>MDKAKRNIKPFDGEKYAIWKFRIRALLAEQDVLKVVDGLMPNEVDDSWKKAERCAKSTIIEYLSDSFLNFATSDITARQILENLDAVYERKSLASQLALRKRLLSLKLSSEMSLLSHFHIFDELISELLAAGAKIEEMDKISHLLITLPSCYDGIITAIETLSEENLTLAFVKNRLLDQEIKIKNDHNDTSKKVMNAIVHNNNNTYKNNLFKNRVTKPKKIFKGNSKYKVKCHHCGREGHIKKDCFHYKRILNNKNKENEKQVQTATSHG[9x]

Here, we show that the Ty1 retrotransposon Copia forms virus-like capsids in vivo and transfers between cells. Copia is enriched at the Drosophila neuromuscular junction (NMJ) and transported across synapses, and disrupting its expression promotes both synapse development and structural synaptic plasticity. Because Copia behaves in a viral-like manner, we used cryogenic-electron microscopy (cryo-EM) to determine the high-resolution structure of the Copia capsid and found that it is distinct from the related dArc1 capsid, with a larger internal capacity and the presence of pores similar to those used by retroviruses to carry out their reverse transcriptase activity. The capsid layer is composed of the Copiagag protein’s CA region, which contains 2 alpha-helical domains.

Our purification protocol enriched capsids of sufficient homogeneity such that we could determine their structure using single-particle cryo-EM methods. Our reconstruction of the Copiagag capsid when enforcing T = 9 icosahedral symmetry reached ~4.2-Å overall resolution. There is a layer of featureless density lining the inner surface of the Copia capsid that likely represents the RNA that comigrates with the Copia-gag protein. Because the RNA does not adopt T = 9 symmetry, its density is amorphous in our reconstruction. The NC region is not clearly visualized in the map but is located in the interior of the capsid and is associated with the density attributed to RNA. The Copia capsid is much larger than that of the T = 4 dArc1 capsid (inner radii of ~220 Å and ~170 Å, respectively), resulting in ~2.2× increased internal capacity. We hypothesize that the Copia capsid is larger than dArc1 because it packages larger cargo, such as the longer Copia mRNA (5 kbp versus 2 kbp) as well as the Copia-encoded enzymes reverse transcriptase and/or integrase. Moreover, the Copia capsid also lacks the spike structures that protrude from the outer surface of the dArc1 capsid. In place of the spikes, the Copia capsid contains positively charged pores at the center of each hexameric or pentameric sub-assembly, similar to HIV. We found that Copia capsid formation requires the presence of RNA, as removing bound RNA using anion-exchange chromatography inhibited capsid assembly.>[10x]APQTITELCSEYRNTQIYTINDKILSYTESMAGKREMVIITFKSGETFQVEVPGSQHIDSQKKAIERMKDTLRITYLTETKIDKLCVWNNKTPNSIAAISMKN

The heat-labile enterotoxin (LT), a homologue of the cholera toxin (CT), is produced by enterotoxigenic Escherichia coli (ETEC). LT and CT belong to the AB5 toxin family, consisting of one A-subunit and five B-subunits. The A-subunit is catalytically active and is anchored to the center of the torus-shaped B-pentamer, which is responsible for the binding to epithelial cells. There are two natural variants of LT, one isolated from human-infecting ETEC (hLT) and one from porcine-infecting ETEC (pLT).

Given the inconclusive results from the SPR analysis presented in Section 2.3, we decided to determine the crystal structure of pLTB in complex with branched LNnH. The structure was obtained after co-crystallization and refined to a resolution of 1.45 Å (R/Rfree = 17.5/20.1). The crystal contained two B-pentamers in the asymmetric unit, giving us access to 10 crystallographically distinct B-subunits. The B-pentamers are positioned “top-to-top”, with the primary binding sites on opposite ends, similarly to recent LTB and CTB structures. The ligand LNnH is present in two of the 10 primary binding sites, on opposite ends of the decamer, and characterized by high-quality electron density. Ligand binding stabilized the 50s loop (residues 51 to 60), which is disordered in all other subunits. The β6-branch is folded back on the reducing end of the sugar, with the β6-glycosidic bond interacting with Arg13. The terminal galactose of the β6-branch is exposed, explaining why substitution can occur at the 2-, 3-, or 4-position. Both ligand binding sites are in close proximity to neighboring molecules in the crystal, with similar contacts in both cases, therefore we cannot exclude that the β6-branch may adopt a different conformation (or be less ordered) in solution.17-HYDROXY-18A-HOMO-19-NOR-17ALPHA-PREGNA-4,9,11-TRIEN-3-ONE 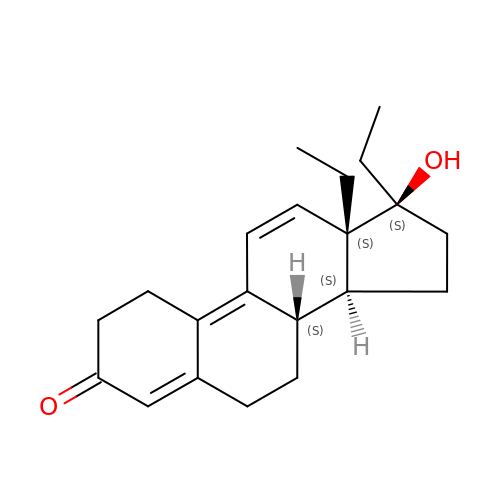| C21 H28 O2 | OXHNQTSIKGHVBH-ANULTFPQSA-N N-{(3R,4S)-4-[(6-amino-4-methylpyridin-2-yl)methyl]pyrrolidin-3-yl}-N'-(3-chlorobenzyl)ethane-1,2-diamine 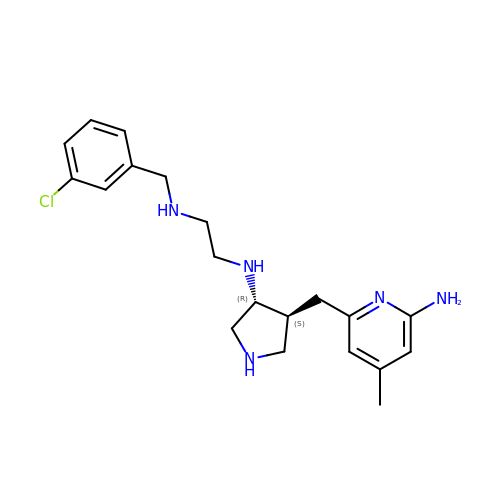| C20 H28 Cl N5 | VWCMAGONQJHIJZ-LPHOPBHVSA-N>[2x]ALPPVAKAAQVVNQTLQLDDSYPDLDSYCRPGASSDYEMQSSDSSWAPFHVVRHHNIPDKVFEHLNAGEVFTKLGLFAEIGYAWASIDSSLFLWDYTHPNPELIGYEEATHTITAVALVPPKPGVFVKTITHVLVVATTSEIILLGVSATPTPSGSKSLTLYSTRMSVHRGGSDVSFIVGTKDGRIFLGGESDTDIHEIFYQQEERWFSSRCGKINHSHPFGSRQQEWLRGLYVDDTRNLLYSLSNRSTIRTYHMEGPEKLTKVIEKDKTSCLRDFAHMADSSPLFTDKTNIVALSPIPATEASKLHLMALTDTGCRLFLSATSSASYTMGGATALAPQSMQLQFVKFPPRESPTRIRTLNGQIIDSQLDKTSRALDPSALGFRFSPGYFFDVVRKHPNQDMLFVSAPDTGRIKVTQPASALKYFEQGTWIELENGNRTIEIGLTTAPFAAAKQPLGFGNELAVQFDQVPGEFAVLTNTGVHIVRRRRLVDIFAKALGNCVSASDDALEREVRKFINQYGRVETIAAALAVACGQGSDLRTGTGRGMDRNTENLARAAFIEYGGQPRLAESDGKQSVSESVRLSSRHDALALYLTRLVRTLWKAKVVQVGSGSDISSTIPTSKLVTIQENVERLRNFLEANKSTIQGLAPPSERLFGRQEDIANQKEHQALHALQKLMESISEGISFVLMLFDERVSDIYARLDAVSQQQLKDLTYEQLFSQTPGKELAKVLVKAIVNRNIASGANVETVADALRRRCGSFCSPDDVVTFKAQEQLQRASEQAHNSPVLRALLAESLRLFEQVAGSLTPANLTTAVEQYISLKYYAGAIQLCLTVAQQKDRGNTALSWVNDGKPANDSRKKAFDERKICYNLIHQVLDKLESDFAGEPELVDGRPTLAATKRMEAYNVVNDSSDEVFHFDLYEWYIEKGWTDRILSIDSPHVITYLQRLAETDFRHAELLCRFYTTRSRFFEAAQVQTNLAKSDLNISLKDRIILLSRAKGNASVNTIGISRQQQQQLNHEASELLEIAHIQDDLLERLVADPRIPEERKAEIEEFLDGPIRTLTDLFNDYADQANYYDLCLLIFHAADFHNPRTILDTWNNLINQSHFEAEQRREYWEIVQAGGDLPAGVIAPIAEPPLPYVYVSQQIQLIAHRTSLDSLIFPVNSLLPVVCAYAINNGQDASIGADPCWPIQLFLNLGVPHALVVQVLENVLDTQEAPFTGRRRKLVVQWIAMAVDMWVREVERRGAMAAAAASGASGSEAVMGSWVSELLGRADQVLTQIAGTGATLRGGAASDAEEIASLRRTVKGLKRSVD;>[2x]DLPPVAKAAQVVNQTLQLDDSYPDLDSYCRPGASSDYEMQSSDSSWAPFHVVRHHNIPDKVFEHLNAGEVFTKLGLFAEIGYAWASIDSSLFLWDYTHPNPELIGYEEATHTITAVALVPPKPGVFVKTITHVLVVATTSEIILLGVSATPTPSGSKSLTLYSTRMSVHRGGSDVSFIVGTKDGRIFLGGESDTDIHEIFYQQEERWFSSRCGKINHSHPFGSRQQEWLRGLYVDDTRNLLYSLSNRSTIRTYHMEGPEKLTKVIEKDKTSCLRDFAHMADSSPLFTDKTNIVALSPIPATEASKLHLMALTDTGCRLFLSATSSASYTMGGATSLAPQSMQLQFVKFPPRESPTRIRTLNGQIIDSQLDKTSRALDPSALGFRFSPGYFFDVVRKHPNQDMLFVSAPDTGRIKVTQPASALKYFEQGTWIELENGNRTIEIGLTTAPFAAAKQPLGFGNELAVQFDQVPGEFAVLTNTGVHIVRRRRLVDIFAKALGNCVSASDDALEREVRKFINQYGRVETIAAALAVACGQGSDLRTGTGRGMDRNTENLARAAFIEYGGQPRLAASDGKQSVSESVRLSSRHDALALYLTRLVRTLWKAKVVQVGSGSDISSTIPTLVTIQENVERLRNFLEANKSTIQGLAPPSERLFGRQEDIANQKEHQALHALQKLMESISEGISFVLMLFDERVSDIYARLDAVSQQQLKDLTYEQLFSQTPGKELAKVLVKAIVNRNIASGANVETVADALRRRCGSFCAPDDVVTFKAQEQLQRASEQAHNAPVLRALLAESLRLFEQVAGSLTPANLTTAVEQMISLKYYAGAIQLCLTVAQQKDRGNTALSWVNDGKPANDSRKKAFDERKICYNLIHQVLDKLESDFAGEPELVDGRPTLAATKRMEAYNVVNDSSDEVFHFDMYEWYIEKGWTDRILSIDSPHVITYLQRLAETDFRHAELLCRFYTTRSRFFEAAQVQTNLAKSDLNISLKDRIILLSRAKGNASVNTIGISRQQQQQLNHEASELLEIAHIQDDLLERLVADPRIPEERKAEIEEFLDGPIRTLTDLFNDYADQANYYDLCLLIFHAADFHNPRTIMDTWNNLINQSHFEAEQRREYWEIVQAGGDLPAGVIAPIAEPPLPYVYVSQQIQLIAHRTSLDSLIFPVNSLLPVVCAYAINNGQDASIGADPCWPIQLFLNLGVPHALMVQVLENVLDTQEAPFTGRRRKLVVQWIAMAVDMWVREVERRGAMAAAAASGASGSEAVMGSWVSELLGRADQVLTQIAGTGATLRGGAASDAEEIASLRRTVKGLKRSVDMLLGGEMARMSFFR;>DLPPVAKAAQVVNQTLQLDDSYPDLDSYCRPGASSDYEMQSSDSSWAPFHVVRHHNIPDKVFEHLNAGEVFTKLGLFAEIGYAWASIDSSLFLWDYTHPNPELIGYEEATHTITAVALVPPKPGVFVKTITHVLVVATTSEIILLGVSATPTPSGSKSLTLYSTRMSVHRGGSDVSFIVGTKDGRIFLGGESDTDIHEIFYQQEERWFSSRCGKINHSHPFGSRQQEWLRGLYVDDTRNLLYSLSNRSTIRTYHMEGPEKLTKVIEKDKTSCLRDFAHMADSSPLFTDKTNIVALSPIPATEASKLHLMALTDTGCRLFLSATSSASYTMGGATALAPQSMQLQFVKFPPRESPTRIRTLNGQIIDSQLDKTSRALDPSALGFRFSPGYFFDVVRKHPNQDMLFVSAPDTGRIKVTQPASALKYFEQGTWIELENGNRTIEIGLTTAPFAAAKQPLGFGNELAVQFDQVPGEFAVLTNTGVHIVRRRRLVDIFAKALGNCVSASDDALEREVRKFINQYGRVETI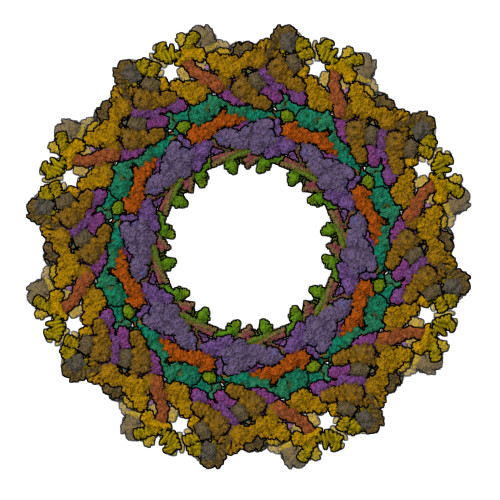AAALAVACGQGSDLRTGTGRGMDRNTENLARAAFIEYGGQPRLAESDGKQSVSESVRLSSRHDALALYLTRLVRTLWKAKVVQVGSGSDISSTIPTSKLVTIQENVERLRNFLEANKSTIQGLAPPSERLFGRQEDIANQKEHQALHALQKLMESISEGISFVLMLFDERVSDIYARLDAVSQQQLKDLTYEQLFSQTPGKELAKVLVKAIVNRNIASGANVETVADALRRRCGSFCSPDDVVTFKAQEQLQRASEQAHNSPVLRALLAESLRLFEQVAGSLTPANLTTAVEQMISLKYYAGAIQLCLTVAQQKDRGNTALSWVNDGKPANDSRKKAFDERKICYNLIHQVLDKLESDFAGEPELVDGRPTLAATKRMEAYNVVNDSSDEVFHFDMYEWYIEKGWTDRILSIDSPHVITYLQRLAETDFRHAELLCRFYTTRSRFFEAAQVQTNLAKSDLNISLKDRIILLSRAKGNASVNTIGISRQQQQQLNHEASELLEIAHIQDDLLERLVADPRIPEERKAEIEEFLDGPIRTLTDLFNDYADQANYYDLCLLIFHAADFHNPRTIMDTWNNLINQSHFEAEQRREYWEIVQAGGDLPAGVIAPIAEPPLPYVYVSQQIQLIAHRTSLDSLIFPVNSLLPVVCAYAINNGQDASIGADPCWPIQLFLNLGVPHALMVQVLENVLDTQEAPFTGRRRKLVVQWIAMAVDMWVREVERRGAMAAAAASGASGSEAVMGSWVSELLGRADQVLTQIAGTGATLRGGAASDAEEIASLRRTVKGLKRSVDMLLGGEMARMSFFR[2x];>[6x]RKAKLLPMEEALLP;>HKKLVINKDMRTDLFSPPN[6x];>[7x]SSLDNIEMAYARQIYIYNEKIVNGHLQPNLVDLCASVAELDDKSISDMWTMVKQMTDVLLTPATDALKNRSSVEVRMEFVRQALAYLEQSYKNYTLVTVFGNLHQAQLGGVPGTYQLVRSFLNIKLPAPLPGLQDGEVEGHPVWALIYYCMRCGDLLAASQVVNRAQHQLGEFKTWFQEYMNSKDRRLSPATENKLRLHYRRALRNNTDPYKRAVYCIIGRCDVTDNQSEVADKTEDYLWLKLNQVCFDDDGTSSPQDRLTLSQFQKQLLEDYGESHFTVNQQPFLYFQVLFLTAQFEAAVAFLFRMERLRCHAVHVALVLFELKLLLKSSGQSAQLLSHEPGDPPCLRRLNFVRLLMLYTRKFESTDPREALQYFYFLRDEKDSQGENMFLRCVSELVIESREFDMILGKLENDGSRKPGVIDKFTSDTKPIINKVASVAENKGLFEEAAKLYDLAKNADKVLELMNKLLSPVVPQISAPQSNKERLKNMALSIAERYRAQGISANKFVDSTFYLLLDLITFFDEYHSGHIDRAFDIIERLKLVPLNQESVEERVAAFRNFSDEIRHNLSEVLLATMNILFTQFKRLKGTSPSSSSRPQRVIEDRDSQLRSQARTLITFAGMIPYRTSGDTNARLVQMEVLMN;>[7x]APPVRSIY;>MATLTDRTYLPPLEDCLTGRTVILSWRLVASALEDADLARLTSPALSTFLRDGFVHELLKHPARVFEPKDLKQEFETKTSSIQTVAPGVDTIKKDALWLADAVAINQVAALRIVLIEYQTRAHSHLVLPLSTQDVANIQEAAGVGDAHASSILSLLNPASAVDAETMWCDFETEARRRERILATYLSERRSFTAAVDALVTFLLHSAPGQHKDLDSLRRALLKDAFAFDEDLDVPDRSKLLTMAPTYMNLVEDCIARAQALPAKLGESFKTEAFELDWLRTAITEAVHSLSIAFQALDLDTPYFAPHELLSEWFELMNSSLFLESILGFEVVADLAMPARSLVSAICLKMLNIDRTIQFLHDFDYPDGEEPYLLSSQTLNKIHTAVTNAVNSGVAASLPVAFAWSLIVHQMHLGYQERAERRDLLVNQRAQAGFELEFQPSASTPNRRRRNSAGSIVSLEASPYDDFLREQRLDNDIAPVEQIAMLATSRGQVYQVMSEMALCLGTTHEAAFRPAVGARARLVFQDLLKRAAYLIPYQDEPVFSLLAILATGRQYWDVTDALSASSLNQVYTDMLDDETLFTQFTMQAINRFPYEFNPFSVLCRVLAAALITNKDKADVVTGWLWRTPTLTVDWNPAWDRSYELCFEDENTNSFRLTRDVDLFGSASPARPRHLAAEERFIIPEGTLGRFVTDVGRTARLEFEHSALALLGKRLEVKAAEEICDSGMAPLDVDEQAEAVAMLATVLRAESLKSTAKGGDPEAPLKFLKEASRLLPHNKDILTVISDTIDGLVEKELLELDGPQIAVLASCLQFLHAALAVCPGRVWAYMSRCALIAGDARPGRLSRITGSLDMYAERFDLLSSAVKLFAALIDSAACSAVQRRAGSTALVSVRSAVENPWLGTSEKILSRVALAIAQAALDVYESTTTWRFRSELDRSILVRDVVGLMHKLVVHAHTLSSHLTSTLSPAAAHIISSFLTPPPSASSLRFQPLLGTLLVALITPRATLYPGQSRILAERVTSVLAFCTSLLRAADFLGQTHIPLQTHLFQSACLLARLPAANAVYRAPVLELLRALVEVAGRAANGSGEPPSLLGYLGSHAARSFISLVEGIDKPFGRVEHAVVTWRFFAAVIRNRQQWMAGCLLTGRTPREALKGGGEQKIERKVGEGSVLAAAMERLREVKSLDVQEAVAVMDFVVSAQNYWPWTIFAVRKEKEVVDALRGYVRGLKAPGMVMKTDGAAAAAFQARIAAYVAETFAMQLYHMRQMRQAEKFAGELVADLDYFLREGVMVWGYNASLHGNFARNFAKRFPGVEVDDFKRTMWLPRELGKGYYYALEVAEQMLGFDAGWGGVKQSGFRKEMETANLNLSLVEAQVSLFHAWEYLLLELTLSLLPKKENAAFARQVLQVVEQCLEANQRSQPPENIFVVLGHARAGLALTLLQRLADANQLPRDVTHLLALVSSAIHAVENPFGANDLPYFRTLLKILFVVLRAAKQGTAKPGESNVAITQQVLTILDRVVARCFRALAALVHEQQQNATDGTTTAPEDLALITAILQACLSVPGIEQCQVQVLNIMAAHDVFQVAVALFSWADRLLPANPSPASSSTSTSATNPASGDPVYGELALLFLLELSALPALAEHLACDGLLGHLAAARLAGYMRRTNVGPFAENAGAARCYAIWAKCLLPLLLNILAALGSTVAPEVAWVLNQFPNLLQSSVERIEPPGFSRPTLSLASTPPRQKFISLLEISEIHSLALLTRVLAACRAQNARDVPEVTWDGAKVLECVEYWLRGRKVLRERLVPLGPREVEWRGMVATGGVVGVAGDGGEGCENRLEEKAVGLLVGVREVLEGGLEGEGE[2x];>DVDTYLSNLQTKTTLSMIADGLERSARDFDAFLEENVTLEWEAQRKRIYQHFG[2x];>EDSILQPGAFSAN[2x];>[5x]MTDLRKLEALQALHAELVAVRQHRFEGLQVLETLLEEQTDAFKALIAKPARDTKDREALGKEPKKLKIGEEEYSLNEDFVNDCLKLADELDLNEKESARILIDCDAEGDVETQSRPLWECGVIRFHQERKYLLDCMRLILEIAADEDIDAGLQESFGVAAEDKIFGIPPPWERNKENQPTQVKKFIPRCMEAMKGVRSMLQCMADKANARNMLQQASLVRPLDNQETLDFSRLSLVEQHECLASILHAAVQRHHATIADFQDFIKILRKWDKYDHFLIHLIPVLAAYITEFGSPEGMGDLQQARRLNDFICKGGDEDSWALPVLGAAVRAWWIAEHNGFYLDDTVQDLRGINLDEEDEQRTKQFLDALKEGAFDFILSVAADCKAQEWQDPSQLGARQWLQRKIPSLPSEPFPFSHFLQHSLMVHLEGFVDATISNLPDVLRKLRTEEDEQRQLRPNHEQDMDLERFLIIISYAYEGRPDAAMSFWEDPDSNLAGFLQWASRRASTPLVSAFCEMLRCLADNEECATAAHNFLLDEGHQASGKMKRSQSLTWSQIFKELEYFTTKVCSERPNPPQASMHRPGRPGADPAEIEPESALMLECYLRLIAKLATESEIARKRLIMDEDFNLVDTILKLSVGVIPHRLRACIFYVLKALMIRKTHEELDAMWRWVEAWMTNPFSSLPGSQGAPQRISFLGQTPGPQECMEMMFREFGTGFEQSNAFIQLLTTLLVPPEGLNSLNDSVPFPEWLGSSIRTLGIEPYVDFVFDVFANRTKDISDPSQLRILRLSCLDFVMVCLVTFNEDLIVLGHESNISIDDAMAATNLATYVRLHPFSRVMEWLFNEKVITSLINTIHQDPISLGSASPDSPLVVSILRAIQVMIKALELQETYLHLVRPEVLRYQGEAGVRRKPVANAAYSAFEDGILSHLSLVVDLGKYCNLGHAELTLACLKLLEKISTSSRILSAWSPDSGRLGHRNKAIVQLERNGEGETISASLSASIMATLDPALAASGENYRVKLAILDFLYACLRATPDQPTIAHQLLGFHCELSKLGIEPKGPFDMQKSLFHSLLNVLITLTVSEEEQGMRGYLVTLKYRVLRILQLLWKSPLSASLVMDELRATNFLFHMLLREVQIQPQLPWDGQLVTGCEFLLSDASLAYIDYLASRAAIFEYIGKELCSVSQNRIPSIKRQIFDALNGQIFVDEEAPLTIPSIFDFFDFINTDYKWEEIPSPHFTYLKDLDLGPCILEHKYAGVHYDIRKAQEILALKRKEYEHSQLATPEFLETVELEEKVLIEWLTVRNRANLLLTARLNLLQAWANLLLVMIESNDFKSTPKMAFLLQALQAILPTLEAFSSLKSDEAFELARVAKVLLWKLDFSQDSDAGLDREQFTVGNLIGDKLFQLFQLCLSAISQCSGTPELRSLYYSICYRYLTAVVDNDATVAATPASSTIGPTRSVTNARARTLKAITLYGDRLLNVICDDAYGSDTTCQTAAMILLNALVHTSRASSAAGVSPADVDCPIIDALNRLNFIGVLVDSLKEILNEWLAPSSTFDPSLSTNASPSLPIPASPSQQYTSAKLALLLQLCQTRQGAKYVLQANLFRALEQSGVFAADPELVEVDSESGVPRVVALERHYALLVALARVVGAAVTARGAHNIVQGRKFLTQHRGLVVHVLKKNAGIGGGVVGNSLASSINGGSTATMTRRDEILAQQALEERIEELAEAFMLLITATGFLEYESEQVPSEQPRAHTTFFH;>SGTGLGEVDVDTYLSNLQTKTTLSMIADGLERSARDFDAFLEENVTLEWEAQRKRIYQHFGIK[5x];>[5x]ILPMYKLSP;>[5x]FG;>[4x]MDEIITRWATDLAKYQKEFKEQAAKVMEWDRLLVENGEKIQKLYTSTYEAERASNEIERQLSNVESQQEELTAWLDRYERELDELYAKQMGSAAGEQAAGPDQERERTYKLAEKLTDQLDEMGKDLAKMIKEINDMSNTLSKGSKPDDPLTQIVRVLNGHLAQLQWIDTNAAALQAKVAAAQK;>[4x]SEALQQEIAKIDEEIQKCIRDKEAVDAFLPAHGEQLAAIPTDVNFVTRKSEGAHNALSSDILAIDQLRELVKQDADNARLSFKAIDNLKLPMQYHQAGLWSKQMGGAGTAGASGASADADGQSNADLISYFSKTADEMEEMMKKFEKTITEIEAHLTGVEAHAMAMQNVAAQSRNAAQGGVDERVYELAAVLREFEESILKVAGVVGGVKEGVTELQLRDFM;>[4x]PIPEQIKLIVDKWNPNHPNCAFKTYLYNKVDEHTVPLYGPGPNEDPKEWEEALQRKPAPNFIPVLCSGFPSIVARLMLQRRVITEFNNKLHQINASLDAILSRHDLDHTVRAFNARRRHAELSRRCLHLAARVQVLRNRGYALSGDEDELKQKLQQIDKTLNDPAQGSRLEELWSRLIVLRGYAEDLKDQINQAGITESDGLGEEIEAKAKKILEDYDKQLQHLKKQVEEAKKDFEEWEKQ;>DEDGLISLIFNKKESDIRGQQQQLVESLHKVLGGHQTLTVNVEGVKTKADNQTEVIIYVVERSPNGTSRRVGASALFSYFEQAHIKANMQSLGVTGAMAQTELSPVQIKQLIQNPL[4x];>[4x]DHLDDSWVTVFGFPQASASYILLQFAQYGNILKHVMSNTGNWMHIRYQSKLQARKALSKDGRIFGESIMIGVKPCIDKSVMESS;>ALFDSLLARNKKQAEGETALGELPSLQLGLADLRQRLRKL[4x];>[4x]MFPAAPSPRTPGTGSRRGPLAGLGPGSTPRTASRKGLPLGSAVSSPVLFSPVGRRSSLSSRGTPTRMFPHHSITESVNYDVKTFGSSLPVKVMEALTLAEVDDQLTINIDEGGWACLVCKEKLIIWKIALSPITKLSVCKELQLPPSDFHWSADLVALSYSSPSGEAHSTQAVAVMVATREGSIRYWPSLAGEDTYTEAFVDSGGDKTYSFLTAVQGGSFILSSSGSQLIRLIPESSGKIHQHILPQGQGMLSGIGRKVSSLFGILSPSSDLTLSSVLWDRERSSFYSLTSSNISKWELDDSSEKHAYSWDINRALKENITDAIWGSESNYEAIKEGVNIRYLDLKQNCDGLVILAAAWHSADNPCLIYYSLITIEDNGCQMSDAVTVEVTQYNPPFQSEDLILCQLTVPNFSNQTAYLYNESAVYVCSTGTGKFSLPQEKIVFNAQGDSVLGAGACGGVPIIFSRNSGLVSITSRENVSILAEDLEGSLASSVAGPNSESMIFETTTKNETIAQEDKIKLLKAAFLQYCRKDLGHAQMVVDELFSSHSDLDSDSELDRAVTQISVDLMDDYPASDPRWAESVPEEAPGFSNTSLIILHQLEDKMKAHSFLMDFIHQVGLFGRLGSFPVRGTPMATRLLLCEHAEKLSAAIVLKNHHSRLSDLVNTAILIALNKREYEIPSNLTPADVFFREVSQVDTICECLLEHEEQVLRDAPMDSIEWAEVVINVNNILKDMLQAASHYRQNRNSLYRREESLEKEPEYVPWTATSGPGGIRTVIIRQHEIVLKVAYPQADSNLRNIVTEQLVALIDCFLDGYVSQLKSVDKSSNRERYDNLEMEYLQKRSDLLSPLLSLGQYLWAASLAEKYCDFDILVQMCEQTDNQSRLQRYMTQFADQNFSDFLFRWYLEKGKRGKLLSQPISQHGQLANFLQAHEHLSWLHEINSQELEKAHATLLGLANMETRYFAKKKTLLGLSKLAALASDFSEDMLQEKIEEMAEQERFLLHQETLPEQLLAEKQLNLSAMPVLTAPQLIGLYICEENRRANEYDFKKALDLLEYIDEEEDININDLKLEILCKALQRDNWSSSDGKDDPIEVSKDSIFVKILQKLLKDGIQLSEYLPEVKDLLQADQLGSLKSNPYFEFVLKANYEYYVQGQI;>[4x]EDRLKIDVIDWLVFDPAQRAEALKQGNAIMRKFLASKKHEAAKEVFVKIPQDSIAEIYNQCEEQGMESPLPAEDDNAIREHLCIRAYLEAHETFNEWFKHMNSVPQKPALIPQPTFTEKVAHEHKEKKYEMDFGIWKGHLDALTADVKEKMYNVLLFVDGGWMVDVREDAKEDHERTHQMVLLRKLCLPMLCFLLHTILHSTGQYQECLQLADMVSSERHKLYLVFSKEELRKLLQKLRESSLMLLDQGLDPLGYEIQ;>YQTERFTKFSDTLKEFKIEQNNEQNPIDPFNIIREFRSAAGQLALDLANSGDESNVISSKDWELEARFWHLVELLLVFRNADLDLDEMELHPYNSRGLFEKKLMQDNKQLYQIWIVMVWLKENTYVMERPKNVPTSKWLNSITSGGLKSCDLDFPLRENTNVLDVKDKEEDHIFFKYIYELILAGAIDEALEEAKLSDNISICMILCGIQEYLNPVIDTQIANEFNTQQGIKKHSLWRRTVYSLSQQAGLDPYERAIYSYLSGAIPNQEVLQYSDWESDLHIHLNQILQTEIENYLLENNQVGTDELILPLPSHALTVQEVLNRVASRHPSESEHPIRVLMASVILDSLPSVIHSSVEMLLDVVKGTEASNDIIDKPYLLRIVTHLAICLDIINPGSVEEVDKSKLITTYISLLKLQGLYENIPIYATFLNESDCL[4x];>DWVEQLILAGSSLRSVFATSKEFDGPCQNEIDLLFSECNDEIDNAKLIMKERRFTASYTFAKFSTGSMLLTKDIVGKSGVSIKRLPTELQRKFLFDDVYLDKEIEKVTIEARKSNPYPQISESSLLFKDALDYMEKTSSDYNLWKLSSILFDPVSYPYKTDNDQVKMALLKKERHCRLTSWIVSQIGPEIEEKIRNSSNEIEQIFLYLLLNDVVRASKLAIESKNGHLSVLISYLGSNDPRIRDLAELQLQKWSTGGCSIDKNISKIYKLLSGSPFEGLFSLKELESEFSWLCLLNLTLCYGQIDEYSLESLVQSHLDKFSLPYDDPIGVIFQLYAANENTEKLYKEVRQRTNALDVQFCWYLIQTLRFNGTRVFSKETSDEATFAFAAQLEFAQLHGHSLFVSCFLNDDKAAEDTIKRLVMREITLLRASTNDHILNRLKIPSQLIFNAQALKDRYEGNYLSEVQNLLLGSSYDLAEMAIVTSLGPRLLLSNNPVQNNELKTLREILNEFPDSERDKWSVSINVFEVYLKLVLDNVETQETIDSLISGMKIFYDQYKHCREVAACCNVMSQEIVSKILEKNNPSIGDSKAKLLELPLGQPEKAYLRGEFAQDLMKCTYKI[4x];>[4x]HNELIHDAVLDYYGKRLATCSSDKTIKIFEVEGETHKLIDTLTGHEGPVWRVDWAHPKFGTILASCSYDGKVLIWKEENGRWSQIAVHAVHSASVNSVQWAPHEYGPLLLVASSDGKVSVVEFKENGTTSPIIIDAHAIGVNSASWAPATIEEDGEHNGTKESRKFVTGGADNLVKIWKYNSDAQTYVLESTLEGHSDWVRDVAWSPTVLLRSYLASVSQDRTCIIWTQDNEQGPWKKTLLKEEKFPDVLWRASWSLSGNVLALSGGDNKVTLWKENLEGKWEPAG;>ILVPMTVNDQPIEKNGDKMPLKFKLGPLSYQNMAFITAKDKYKLYPVRIPRLDTSKEFSAYVSGLFEIYRDLGDDRVFNVPTIGVVNSNFAKEHNATVNLAMEAILNELEVFIGRVKDQDGRVNRFYELEESLTVLNCLRTMYFILDGQDVEENRSEFIESLLNWINRSDGEPDEEYIEQVFSVKDSTAGKKVFETQYFWKLLNQLVLRGLLSQAIGCIERSDLLPYLSDTCAVSFDAVSDSIELLKQYPKDSSSTFREWKNLVLKLSQAFGSSATDISGELRDYIEDFLLVIGGNQRKILQYSRTWYESFCGFLLYYIPSLELSAEYLQMSLEANVVDITNDWEQPCVDIISGKIHSILPVMESLDSCTAAFTAMICEAKGLIENIFEGEKNSDDYSNEDNEMLEDLFSYRNGMASYMLNSFAFELCSLGDKELWPVAIGLIALSATGTRSAKKMVIAELLPHYPFVTNDDIEWMLSICVEWRLPEIAKEIYTTLGNQMLSAHNIIESIANFSRAGKYELVKSYSWLLFEASCMEGQKLDDPVLNAIVSKNSPAEDDVIIPQDILDCVVTNSMRQTLAPYAVLSQFYELRDREDWGQALRLLLLLIEFPYLPKHYLVLLVAKFLYPIFLLDDKKLMDEDSVATVIEVIETKWDDADEKSSNLYETIIEADKSLPSSMATLLKNLRKKLNFKLCQAFM[4x];>MQPFDSGHDDLVHDVVYDFYGRHVATCSSDQHIKVFKLDKDTSNWELSDSWRAHDSSIVAIDWASPEYGRIIASASYDKTVKLWEEDPDQEECSGRRWNKLCTLNDSKGSLYSVKFAPAHLGLKLACLGNDGILRLYDALEPSDLRSWTLTSEMKVLSIPPANHLQSDFCLSWCPSRFSPEKLAVSALEQAIIYQRGKDGKLHVAAKLPGHKSLIRSISWAPSIGRWYQLIATGCKDGRIRIFKITEKLSPLASEESLTNSNMFDNSADVDMDAQGRSDSNTEEKAELQSNLQVELLSEHDDHNGEVWSVSWNLTGTILSSAGDDGKVRLWKATYSNEFKCMSVIT[4x];>ACLSRIDANLLQYYEKPEPNNTVDLYVSNNSNNNGLKEGDKSISTPVPQPYGSEYSNCLLLSNSEYICYHFSSRSTLLTFYPLSDAYHGKTINIHLPNASMNQRYTLTIQEVEQQLLVNVILKDGSFLTLQLPLSFLFSSANTLNGEWFHLQNPYDFTVRVPHFLFYVSPQFSVVFLEDGGLLGLKKVDGVHYEPLLFNDNSYLKSLTRFFSRSSKSDYDSVISCKLFHERYLIVLTQNCHLKIWDLTSFTLIQDYDMVSQSDSDPSHFRKVEAVGEYLSLYNNTLVTLLPLENGLFQMGTLLVDSSGILTYTFQNNIPTNLSASAIWSIVDLVLTRPLELNVEASYLNLIVLWKSGTASKLQILNVNDESFKNYEWIESVNKSLVDLQSEHDLDIVTKTGDVERGFCNLKSRYGTQIFERAQQILSENKIIMAHNEDEEYLANLETILRDVKTAFNEASSITLYGDEIILVNCFQPYNHSLYKLNTTVENWFYNMHSETDGSELFKYLRTLNGFASTLSNDVLRSISKKFLDIITGELPDSMTTVEKFTDIFKNCLENQFEITNLKILFDELNSFDIPVVLNDLINNQMKPGIFWKKDFISAIKFDGFTSIISLESLHQLLSIHYRITLQVLLTFVLFDLDTEIFGQHISTLLDLHYKQFLLLNLYRQDKCLLAEVLLKDSSEFSFGVKFFNYGQLIAYIDSLNSNVYNASITENSFFMTFFRSYIIENTSHKNIRFFLENVECPFYLRHNEVQEFMFAMTLFSCGNFDQSYEIFQLHDYPEAINDKLPTFLEDLKSENYHGDSIWKDLLCTFTVPYRHSAFYYQLSLLFDRNNSQEFALKCISKSAEYSLKEIQIEELQDFKEKQHIHYLNLLIHFRMFEEVLDVLRLGHECLSDTVRTNFLQLLLQEDIYSRDFFSTLLRLCNAHSDNGELYLRTVDIKIVDSILSQNLRSGDWECFKKLYCFRMLNKSERAAAEVLYQYILMQADLDVIRKRKCYLMVINVLSSFDSAYDQWILNGSKVVTLTDLRDELRG[4x];>[4x]MEEIYAKFVSQKISKTRWRPLPPGSLQTAETFATGSWDNEENYISLWSIGDFGNLDSDGGFEGDHQLLCDIRHHGDVMDLQFFDQERIVAASSTGCVTVFLHHPNNQTLSVNQQWTTAHYHTGPGSPSYSSAPCTGVVCNNPEIVTVGEDGRINLFRADHKEAVRTIDNADSSTLHAVTFLRTPEILTVNSIGQLKIWDFRQQGNEPSQILSLTGDRVPLHCVDRHPNQQHVVATGGQDGMLSIWDVRQGTMPVSLLKAHEAEMWEVHFHPSNPEHLFTCSEDGSLWHWDASTDVPEKSSLFHQGGRSSTFLSHSISNQANVHQSVISSWLSTDPAKDRIEITSLLPSRSLSVNTLDVLGPCLVCGTDAEAIYVTRHLFS;>[4x]SNQYQLPLNVRPYTTTWCSQSPSCSNLLAIGHDTGITIYCASEEQTPGSTGLTLQELFTIQTGLPTLHLSFSSSCSYSENLHDGDGNVNSSPVYSLFLACVCQDNTVRLIITKNETIITQHVLGGKSGHHNFVNDIDIADVYSADNRLAEQVIASVGDDCTLIIWRLTDEGPILAGYPLSSPGISVQFRPSNPNQLIVGERNGNIRIFDWTLNLSAEENSQTELVKNPWLLTLNTLPLVNTCHSSGIASSLANVRWIGSDGSGILAMCKSGAWLRWNLFANNDYNEISDSTMKLGPKNLLPNVQGISLFPSLLGACPHPRYMDYFATAHSQHGLIQLINTYEKDSNSIPIQLGMPIVDFCWHQDGSHLAIATEGSVLLTRLMGFT>[6x]MAYETIIVEVEDHVALITLNRPDALNALNDQLLSELVKALEDAQNNDKVRCIVITGSEKAFAAGADIKMMSEKSFVDVFAGDLFGPEAEGIMRIRKPIIAAVSGYALGGGCELAMMCDFIICSDTAKFGQPEINLGVIAGMGGSQRLTRFIGKSKSMDMNLTGRFMDAEEAERSGLVSRVVPAKKLMEETMTA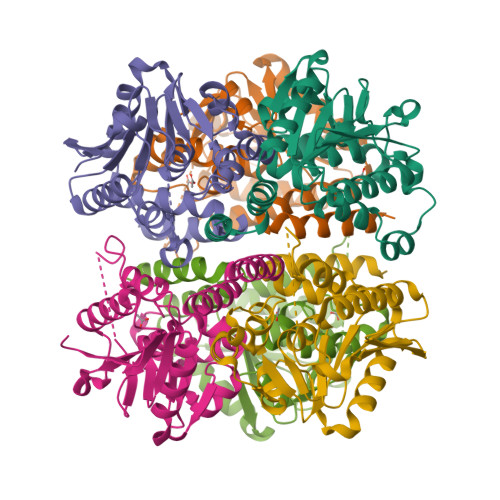AQKIAEKSMIAVMAVKEAVNRSYEVPLREGLLFERRVFQSLFATEDQKEGMSAFAEKREAQFRDK> MSLSVAEKSYLYDSLASTPSIRPDGRLPHQFRPIEIFTDF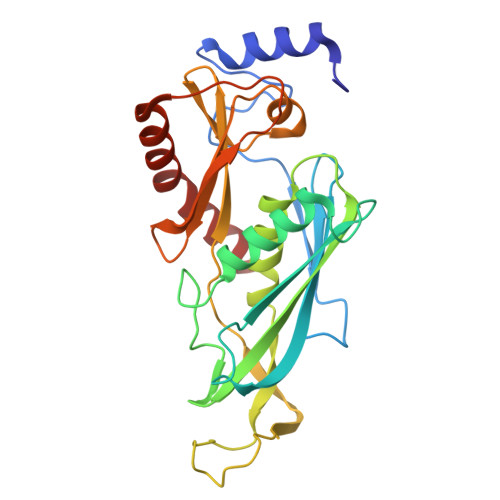LPSSNGSSRIIASDGSECIVSIKSKVVDHHVENELLQVDVDIAGQRDDALVVETITSLLNKVLKSGSGVDSSKLQLTKKYSFKIFVDVLVISSHSHPISLISFAIYSALNSTYLPKLISAFDDLEVEELPTFHDYDMVKLDINPPLVFILAVVGNNMLLDPAANESEVANNGLIISWSNGKITSPIRSVALNDSNVKSFKPHLLKQGLAMVEKYAPDVVRSLENL TNF-receptor associated factor (TRAF) proteins are key intracellular signaling molecules in the tumor necrosis receptor (TNFR) and toll like receptor (TLR) family signaling pathways that play critical roles in the immune system. TRAF1 is a well-known adaptor molecule that regulates the activation of NF-kappaB and JNK1516. TRAF1 is considered a unique family among TRAFs in that it lacks the N-terminal RING finger domain that is critical for relaying the signal to downstream effectors. The TRAF domain, which is composed of 7–8 anti-parallel β-strand folds followed by a coiled-coil region that mediates protein interactions, usually forms mushroom-like trimeric structures in solution.

The 2.8 Å crystal structure of the TRAF domain (corresponding to amino acids 220–416) consisting of the TRAF-N coiled-coil domain and the TRAF-C anti-parallel β-sandwich domain was solved using the molecular replacement (MR) method and refined to Rwork = 21.0% and Rfree = 26.2%. There was one trimer (three monomers) in the asymmetric unit, chain A, chain B, and chain C, and three molecules related by near perfect three-fold symmetry. The structure of the TRAF1 TRAF domain revealed that TRAF-C comprises two α-helices (α1–α2) and six β-sheets (β1–β8). β2 and β7, which have been shown at other TRAF structures, were not detected and were replaced by the loop structure in the TRAF1 structure. The structure of the trimeric TRAF1 TRAF domain exhibited a typical mushroom shape, in which the TRAF domain forms the cap and the coiled-coil domain forms the stalk. The trimeric TRAF-C domains were loosely packed with the narrow portion of the binding interface, while the TRAF-N coiled-coil domain was tightly packed with massive hydrophobic interactions and salt bridges. The trimeric interface of the TRAF1 TRAF-N coiled-coil domain is primarily formed by several hydrophobic patches and two salt bridge clusters. The major force for formation of the trimeric interfaces of the TRAF1 TRAF-C domain was several hydrogen bonds formed between Glu261, Leu270 and Lys272 from one TRAF molecule (chain B) and Lys300, Tyr301, Glu332 and Tyr333 from the second molecule (chain A). Analysis by size-exclusion chromatography and MALS indicated that the TRAF1 TRAF domain exists as a trimer in solution, while the TRAF1 TRAF-C domain without the TRAF-N coiled-coil domain exists as a monomer in solution, indicating that the TRAF-N coiled-coil domain is critical for trimer formation of TRAF1. Pair-wise structural alignments between the TRAF1 TRAF domain and other TRAF domains showed that the position and length of several loops in the TRAF1 TRAF domain differed from those of other TRAF domains. Finally, we produced F325D, S368R, and R308D mutations to analyse the interaction sites on TRAF1 and performed ITC.

>HQSQLDRERILSLEQRVVELQQTLAQKDQALGKLEQSLRLMEEASFDGTFLWKITNVTRRCHESACGRTVSLFSPAFYTAKYGYKLCLRLYLNGDGTGKRTHLSLFIVIMRGEYDALLPWPFRNKVTFMLLDQNNREHAIDAFRPDLSSASFQRPQSETNVASGCPLFFPLSKLQSPKHAYVKDDTMFLKCIVETST[3x]>[6x]GSHMSKSDVFHLGLTKNDLQGATLAIVPGDPDRVEKIAALMDKPVKLASHREFTTWRAELDGKPVIVCSTGIGGPSTSIAVEEL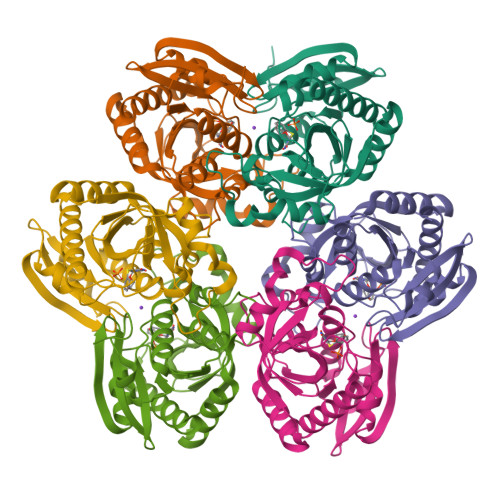AQLGIRTFLRIGTTGAIQPHINVGDVLVTTASVRLDGASLHFAPLEFPAVADFECTTALVEAAKSIGATTHVGVTASSDTFYPGQERYDTYSGRVVRHFKGSMEEWQAMGVMNYEMESATLLTMCASQGLRAGMVAGVIVNRTQQEIPNAETMKQTESHAVKIVVEAARRLL>MVNVAVIGAAGGIGQSLSLLLLRELPFGSTLSLYDVVGAPGVAADLSHIDRAGITVKHAAGKLPPVPRDPALTELAEGVDVFVIVAGVPRKPGMTRDDLFNVNAGIVMDLVLTCASVSPNACFCIVTNPVNSTTPIAAQTLRKIGVYNKNKLLGVSLLDGLRATRFINNARHPLVVPYVPVVGGHSDVTIVPLYSQIPGPLPDESTLKEIRKRVQVAGTEVVKAKAGRGSATLSMAEAGARFTMHVVKALMGLDTPMVYAYVDTDGEHECPFLAMPVVLGKNGIERRLPIGPITTVEKEMLEEAVGVVKKNIAKGETFARSKL[4x];>[2x]MDCSTGAAIGQQFAKDAFHMHGGVGVGPTGNSEHDVLMNEMMMVQTPTGPAGEWTHQFAAYQGQQQQQQQQHPQELAMRHQQNDAFMLRQQQEMEEAFCTFCTTHPHSHAHSHQPQGLVGPAMMGPQIMPPMMFGPGTGGFMMGAPPMMPYASMKFAGDAAMAAANNTNMTQGATATSTTSVQQELQQQSSDNGWVEKLRDAEWAQDYSDAQVFTLEGQSEQTMEEHAKNSEFYQFMDKIRSKELLIDEETGQLVQGPGPDPDAPEDAEYLKEWAAAEGLNMPPGFFEHMMQRPQGNNEQAEGRLFDGSNDALMDDGALDNAADVEEWVREYAEAQEQLQRV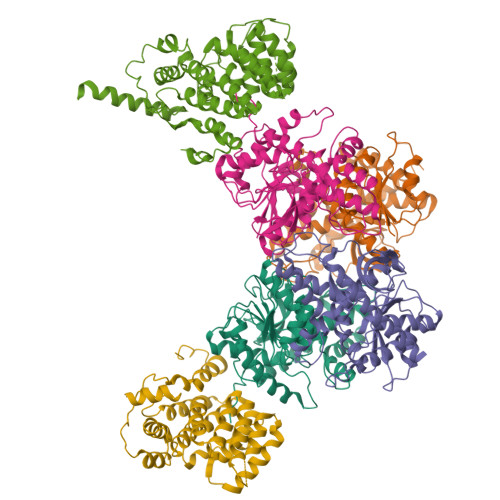QNETNYPFEPNNPYMYHDKPMEEGIAMLQLANMAEAALAFEAVCQKEPENVEAWRRLGTTQAENEKDCLAIIALNHARMLDPKDIAVHAALAVSHTNEHNVGAALQSLRSWLLSQPQYEHLGLVDLREVAADEGLDEVPEENYFFAAPSEYRDCCTLLYAAVEMNPNDPQLHASLGVLHNLSHRFDEAAKNFRRAVELRPDDAHMWNKLGATLANGNRPQEALEAYNRALDINPGYVRVMYNMAVSYSNMAQYPLAAKHITRAIALQAGGTNPQGEGSRIATRGLWDLLRMTLNLMDRSDLVEASWQQDLTPFLREFGLEEMAV>[24x]MGSSHHHHHHSQDPMLPLTLLNATQGRPILV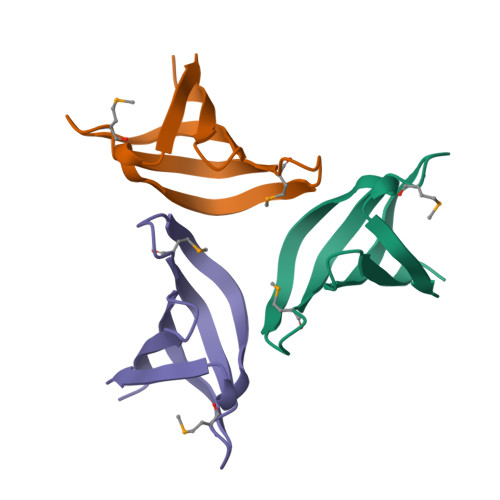ELKNGETFNGHLENCDNYMNLTLREVIRTMPDGDKFFRLPECYIRGNNIKYLRIQDEVLSQVAKQQAQQRENRG>GNASSIVQTINVTGDGNVFKPSAETSSTAVPSLSLSPGMLN[10x];> MANVWGVRLADSLSSPTIETRTRQYTLHDLCSDLDANPGREPWKPLRNQRTNNIVAVQLFRPLQGLVLDTQLYGFPGAFDDWERFMREKLRVLKYEVLRIYPISNYSNEHVNVFVANALVGAFLSNQAFYDLLPLLIINDTMIGDLLGTGASLSQFFQSHGDVLEVAAGRKYLQMENYSNDDDDPPLFAKDLSDYAKAFYSDTYEVLDRFFWTHDSSAGVLVHYDKPTNGHHYLLGTLTQMVSAPPYIINATDAMLLESCLEQFSANVRARPAQPVTRLDQCYHLRWGAQYVGEDSLTYRLGVLSLLATNGYQLARPIPRQLTNRWLSSFVSQIMSDGVNETPLWPQERYVQIAYDSPSVVDGATQYGYVRKNQLRLGMRISALQSLSDTPSPVQWLPQYTIDQAAMDEGDLMVSRLTQLPLRPDYGNIWVGDALSYYVDYNRSHRVVLSSELPQLPDTYFDGDEQYGRSLFSLARKIGDRSLVKDTAVLKHAYQAIDPNTGKEYLRSGQSVAYFGASAGHSGADQPLVIEPWIQGKISGVPPPSSVRQFGYDVARGAIVDLARPFPSGDYQFVYSDVDQVVDGHDDLSISSGLVESLLSSCMHATAPGGSFVVKINFPTRPVWHYIEQKILPNITSYMLIKPFVTNNVELFFVAFGVHQHSSLTWTSGVYFFLVDHFYRYETLSTISRQLPSFGYVDDGSSVTGIETISIENPGFSNMTQAARIGISGLCANVGNARKSIAIYESHGARVLTITSRRSPASARRKSRLRYLPLIDPRSLEVQARTILPADPVLFENVSGASPHVCLTMMYNFEVSSAVYDGDVVLDLGTGPEAKILELIPATSPVTCVDIRPTAQPSGCWNVRTTFLELDYLSDGWITGVRGDIVTCMLSLGAAAAGKSMTFDAAFQQLIKVLSKSTANVVLVQVNCPTDVVRSIKGYLEIDSTNKRYRFPKFGRDEPYSDMDALEKICRTAWPNCSITWVPLSYDLRWTRLALLESTTLSSASIRIAELMYKYMPIMRIDIHGLPMEKRGNFIVGQNCSLVIPGFNAQDVFNCYFNSALAFSTEDVNAAMIPQVSAQFDATKGEWTLDMVFSDAGIYTMQALVGSNANPVSLGSFVVDSPDVDITDAWPAQLDFTIAGTDVDITVNPYYRLMTFVRIDGQWQIANPDKFQFFSSASGTLVMNVKLDIADKYLLYYIRDVQSRDVGFYIQHPLQLLNTITLPTNEDLFLSAPDMREWAVKESGNTICILNSQGFVLPQDWDVLTDTISWSPSIPTYIVPPGDYTLTPL;>[10x]PGGVPWIAVGDETSVTSPGALRRMTSKDIPETAIINTDNSSGAVPSESALVPYIDEPLVVVTEHAITNFTKAEMALEFNREFLDKMRVLSVSPKYSDLLTYVDCYVGVSARQALNNFQKQVPVITPTRQTMYVDSIQAALKALEKWEIDLRVAQTLLPTNVPIGEVSCPMQSVVKLLDD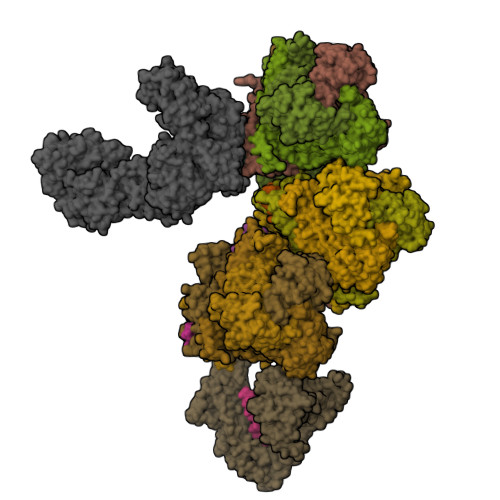QLPDDSLIRRYPKEAAVALAKRNGGIQWMDVSEGTVMNEAVNAVAASALAPSASAPPLEEKSKLTEQAMDLVTAAEPEIIASLVPVPAPVFAIPPKPADYNVRTLRIDEATWLRMIPKSMNTPFQIQVTDNTGTNWHLNLRGGTRVVNLDQIAPMRFVLDLGGKSYKETSWDPNGKKVGFIVFQSKIPFELWTAASQIGQATVVNYVQLYAEDSSFTAQSIIATTSLAYNYEPEQLNKTDPEMNYYLLATFIDSAAITPTNMTQPDVWDALLTMSPLSAGEVTVKGAVVSEVVPADLIGSYTPESLNTSLPNDAARCMIDRASKIAEAIKIDDDAGPDEYSPNSVPIQGQLAISQLETGYGVRIFNPKGILSKIASRAMQAFIGDPSTIITQAAPVLSDKNNWIALAQGVKTSLRTKSLSAGVKTAVSKLSSSESIQNWTQGFLDKVSAHFPAPKPDCPTSGDSGESSNRRVKRDSYAGVVKRGYTR(2R)-N-methylmorpholine-2-carboxamide 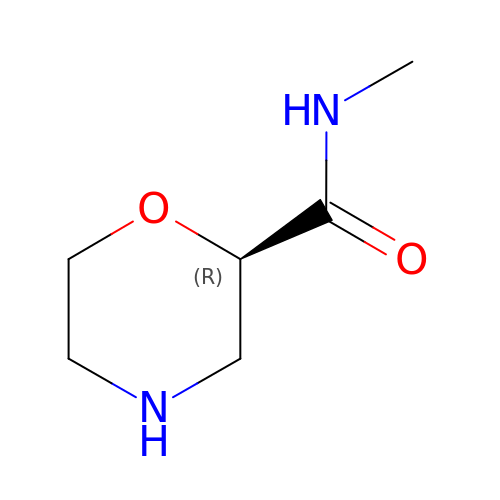| C6 H12 N2 O2 | JOFDGSQZWZFPJC-RXMQYKEDSA-N>[17x]GANPTTAETLDATRRVDDATVAIRSAINNL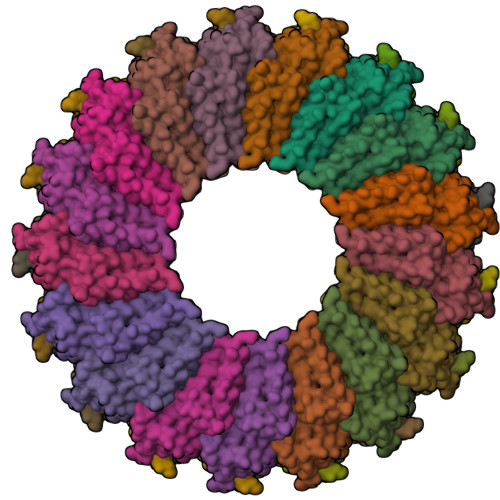IVELIRGTGSYNRSSFESSSGLVWTSGPAGEGSYSITTPSQFVFLSSAWADPIELINLCTNALGNQFQTQHARTVVQRQFSEVWKPSPQVTVRFPDSDFKVYRYNAVLDPLVTALLGAFDTRNRIIEVENQ> DKPVAHVVANHQVEEQLEWLSQRANALLANGMDLKDNQLVVPADGLYLVYSQVLFKGQGCPDYVLLTHTVSRFAISYQ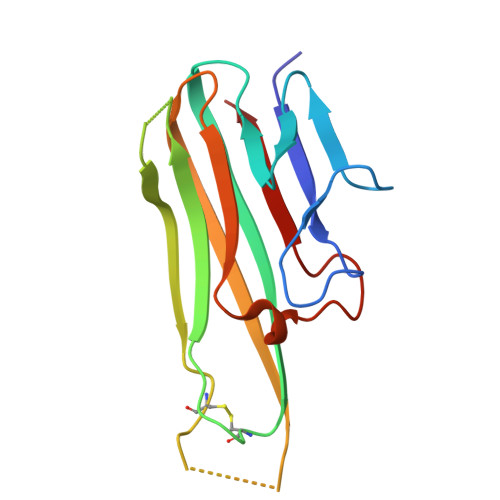EKVNLLSAVKSPCPKDTPEGAELKPWYEPIYLGGVFQLEKGDQLSAEVNLPKYLDFAESGQVYFGVIAL> MSATKSIVGEALEYVNIGLSHFLALPLAQRISLIIIIPFIYNIVWQLLYSLRKDRPPLVFYWIPWVGSAVVYGMKPYEFFEECQKKYGDIFSFVLLGRVMTVYLGPKGHEFVFNAKLADVSAEAAYAHLTTPVFGKGVIYDCPNSRLMEQKKFVKGALTKEAFKSYVPLIAEEVYKYFRDSKNFRLNERTTGTIDVMVTQPEMTIFTASRSLLGKEMRAKLDTDFAYLYSDLDKGFTPINFVFPNLPLEHYRKRDHAQKAISGTYMSLIKERRKNNDIQDRDLIDSLMKNSTYKDGVKMTDQEIANLLIGVLMGGQHTSAATSAWILLHLAERPDVQQELYEEQMRVLDGGKKELTYDLLQEMPLLNQTIKETLRMHHPLHSLFRKVMKDMHVPNTSYVIPAGYHVLVSPGYTHLRDEYFPNAHQFNIHRWNNDSASSYSVGEEVDYGFGAISKGVSSPYLPFGGGRHRCIGEHFAYCQLGVLMSIFIRTLKWHYPEGKTVPPPDFTSMVTLPTGPAKIIWEKRNPEQKIGGRHHH

The fungal cytochrome P450 lanosterol 14α-demethylase (CYP51) is required for the biosynthesis of fungal-specific ergosterol and is the target of azole antifungal drugs. The azoles target the cytochrome P450 enzyme lanosterol 14α-demethylase (CYP51), a key enzyme in the ergosterol biosynthetic pathway. The tetrazole antifungals are a new generation of azoles designed to overcome the toxicity and drug interactions present in imidazole and triazoles. The CYP51 LBP comprises a heme at the base of the active site, a substrate entry channel and a putative product exit channel.

In this study, we report the X-ray crystal structure of VT-1129 (quilseconazole) in complex with S. cerevisiae CYP51 (ScCYP51) as a surrogate to understand the molecular basis of CpCYP51 susceptibility to tetrazoles. As we are currently unable to obtain diffracting crystals of CpCYP51-6×His, we have used instead ScCYP51-6×His as a surrogate to investigate the binding of azole drugs. The structure includes the full protein sequence from isoleucine 7 (I7) to the first histidine of the C-terminal hexa-histidine tag, most of the N-terminal membrane-associated helix, the transmembrane domain and the catalytic domain, including the fungus-specific loop. Strong electron density within the active site allowed modelling of VT-1129. The ligand occupied the sixth axial (distal) coordination site with the heme iron via either the N-3 or N-4 atom of the tetrazole ring, at a distance of 2.1 Å. There are 20 residues within 4 Å of VT-1129. Unexpectedly, the water mediating the hydrogen bond network previously seen between the heme ring C propionate carboxyl (RCC), the Y140 residue and the tertiary hydroxyl group in VT-1161 or the triazoles FLC or VCZ was not observed in the complex with VT-1129, although there is some evidence of density at the position of the water. In the absence of water, the Y140 hydroxyl forms a short hydrogen bond only with the heme RCC. The tail of VT-1129 lies in the substrate entry channel. However, our studies with full-length ScCYP51 show that neither VT-1161 nor VT-1129 are likely to form hydrogen bonds with the homologous residue H381.> MSSSHK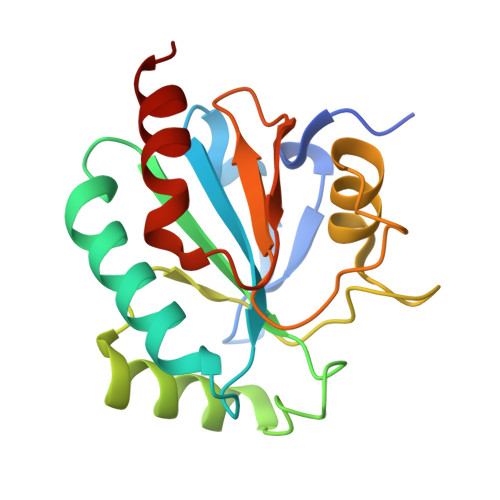SWNSIYEFTVKDINGVDVSLEKYRGHVCLIVNVACKSGATDKNYRQLQEMHTRLVGKGLRILAFPCNQFGGQEPWAEAEIKKFVTEKYGVQFDMFSKIKVNGSDADDLYKFLKSRQHGTLTNNIKWNFSKFLVDRQGQPVKRYSPTTAPYDIEGDIMELLEKK>[2x]SNAMTSTDSITSAPDAALAAVAALPARIVAAWADHDADRFADVFAEDGTMILPGLFRKGRENIRTHMAAAFAGPYKGTRVIGSPIDARLLGDGIALLITEG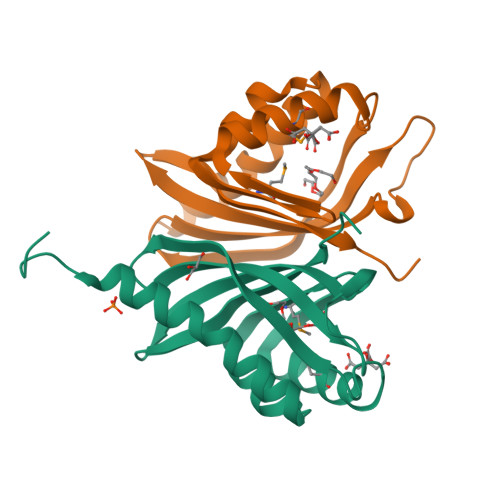GILAPGETEASGDGAVRASWLAVEQDGQWRLAAYQNSPRGND> MNLVLMGLPGAGKGTQGERIVEDYGIPHISTGDMFRAAMKEETPLGLEAKSYIDKGELVPDEVTIGIVKERLGKDDCERGFLLDGFPRTVA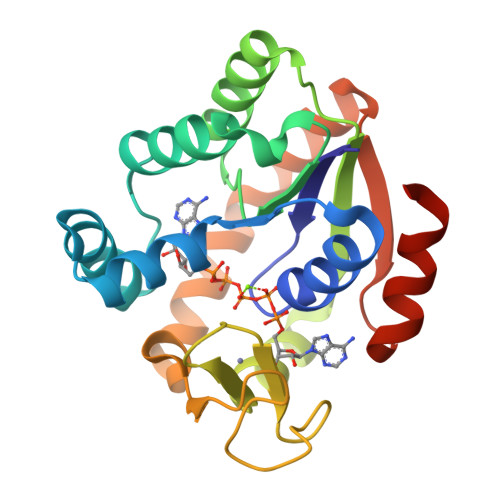QAEALEEILEEYGKPIDYVINIEVDKDVLMERLTGRRICSVCGTTYHLVFNPPKTPGICDKDGGELYQRADDNEETVSKRLEVNMKQTQPLLDFYSEKGYLANVNGQQDIQDVYADVKDLLGGLKK>[2x]GSHMATVSVFPGARLLTIGDANGEIQRHAEQQALR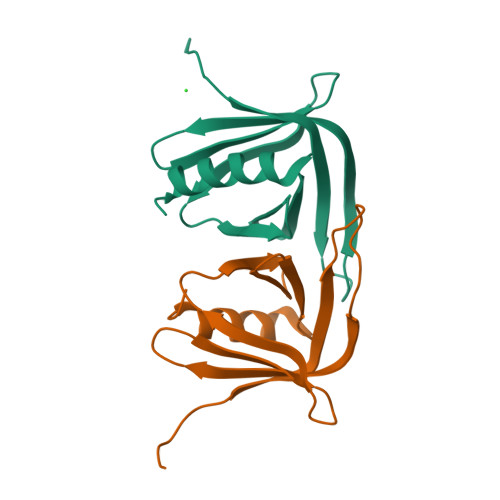LEVRAGPDAAGIALYSHEDVCVFKCSVSRETECSRVGRQSFIITLGCNSVLIQFATPHDFCSFYNILKTCRGHTLERSVFSE> MSQEALKAPVVVLGAGLASVSFVAELRQAGYQGLITVVGDEAERPYDRPPLSKDFMAHGDAEKIRLDCKRAPEVEWLLGVTAQSFDPQAHTVALSDGRTLPYGTLVLATGAAPRALPTLQGATMPVHTLRTLEDARRIQAGLRPQSRLLIVGGGVIGLELAATARTAGVHVSLVERQPRLMSRAAPATLADFVARYHAAQGVDLRFERSVTGSVDGVVLLDDGTRIAADMVVVGIGVLANDALARAAGLACDDGIFVDAYGRTTCPDVYALGDVTRQRNPLSGRFERIETWSNAQNQGIAVARHLVD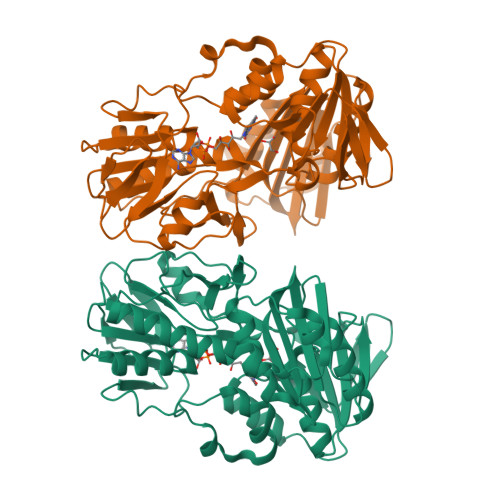PTAPGYAELPWYWSDQGALRIQVAGLASGDEEIVRGEVSLDAPKFTLIELQKGRIVGATCVNNARDFAPLRRLLAVGAKPDRAALADPATDLRKLAAAVAA Human mitochondrial nuclease EXOG (hEXOG) is important for mtDNA integrity. hEXOG depletion selectively increases lesions in mtDNA, but has no effect on chromosomal DNA. Human EXOG shares sequence homology with members of ββα-Me nuclease family, which contains nonspecific endonucleases. The catalytic Core domain of hEXOG is identical to EndoG, but its C-terminal extension forms a unique Wing domain that converts the enzyme from a nonspecific endonuclease into a DNA-geometry-specific exonuclease. Conversely, in mitochondrial LP-BER, the nuclease reaction occurs before DNA synthesis: hEXOG processes the 5′-end of DNA downstream of the lesion, generating an optimal substrate for DNA synthesis catalysed by Pol γ.

The nuclease-deficient variant, hEXOG–H140A, was refolded and purified similarly to wild type and used for co-crystallization with a 10 bp DNA. Successful crystallization experiments were performed at enzyme concentrations greatly exceeding the Kd value for the weaker DNA-binding site of the hEXOG dimer as determined by ITC; consequently, DNA occupied both active sites. Both DNA duplexes are oriented such that the 5′-P end of the substrate is proximal and the 5′-OH end is distal to the active site. However, the two Wing domains undergo different conformational changes from their positions in the apo structure: one rotates only 3°, whereas the other rotates 35° away from the DNA. Consequently, upon DNA binding, hEXOG becomes asymmetrical where one active site remains in the ‘closed' configuration and the other becomes ‘open'. The dsDNA is bound to each positively charged active site cleft; the substrate strand interacts primarily with the Core domain and the complementary strand with the Wing domain, explaining why the Wing domain of hEXOG increases specificity for dsDNA. In the closed active site, the complementary strand interacts with Wing residues R314, R315, R320, R324 and K327, with R324 forming a bipartite interaction with the +3 nt DNA backbone at distances of 3.1 and 3.4 Å; R315 and K327 are, respectively, 4.3 and 6.7 Å from the +2 nt DNA backbone. In the open active site, the complementary DNA strand lacks several interactions, because the bipartite distances to R324 are increased threefold (to 9.4 and 9.8 Å), and R315 and K327 are similarly displaced (10.2 and 16.4 Å, respectively) from the +2 nt backbone. The nature of Mg2+ was confirmed by Mn2+ substitution and single-wavelength anomalous dispersion data.

>MKAVLEQFGFPLTGTEARCYTNHALSYDQAKRVPRWVLEHISKSKIMGDADRKHCKFKPDPNIPPTFSAFNEDYVGSGWSRGAMAPAGNNKFSSKAMAETFYLSNIVPQDFDNNSGYWNRIEMYCRELTERFEDVWVVSGPLTLPQTRGDGKKIVSYQVIGEDNVAVPSHLYKVILARRSSVSTEPLALGAFVVPNEAIGFQPQLTEFQVSLQDLEKLSGLVFFPHLDRTSDIRNICSVDTCKLLDFQEFTLYLSTRKIEGARSVLRLEKIMENLKNAEIEPDDYFMSRYEKKLEELKAKEQSGTQIRKPSHHHHHH[2x]>MLNTTFANAKFANPFMNASGVHCMTIEDLEELKASQAGAYITKSSTLEKREGNPLPRYVDLELGSINSMGLPNLGFDYYLDYVLKN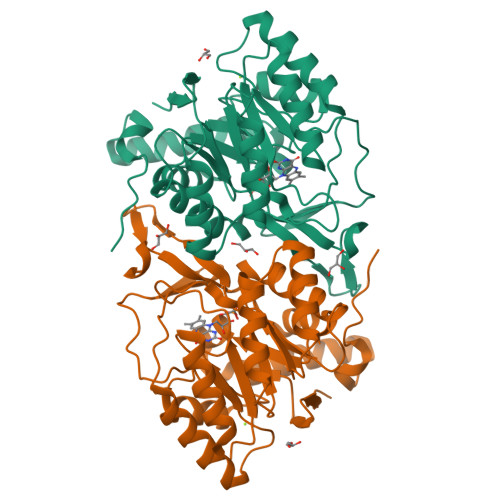QKENAQEGPIFFSIAGMSAAENIAMLKKIQESDFSGITELNLSCPNVPGEPQLAYDFEATEKLLKEVFTFFTKPLGVKLPPYFDLVHFDIMAEILNQFPLTYVNSVNSIGNGLFIDPEAESVVIKPKDGFGGIGGAYIKPTALANVRAFYTRLKPEIQIIGTGGIETGQDAFEHLLCGATMLQIGTALHKEGPAIFDRIIKELEEIMNQKGYQSIADFHGKLKSL[2x]> MADKELKFLVVDDFSTMRRIVRNLLKELGFNNVEEAEDGVDALNKLQAGGFGFIISDWNMPNMDGLELLKTIRADSAMSALPVLMVTAEAKKE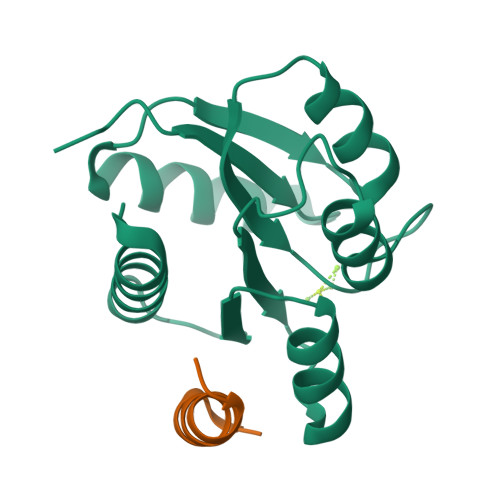NIIAAAQAGASGYVVKPFTAATLEEKLNKIFEKLGM;> XASQDQVDDLLDSLGF> MSHHHHHHVSKIFFEQGTYQCLENCGTVALTIIRRGGDLTNTVFVDFRTEDGTANAGSDYEFTEGTVVFKPGETQKEIRVGIIDDDIFEEDKNFLVHLSNVKVSSEASEDGILEANHVSALACLGSPSTATVTIFDDDHAGIFTFEEPVTHVSESIGIMEVKVLRTSGARGNVIVPYKTIEGTARGGGEDF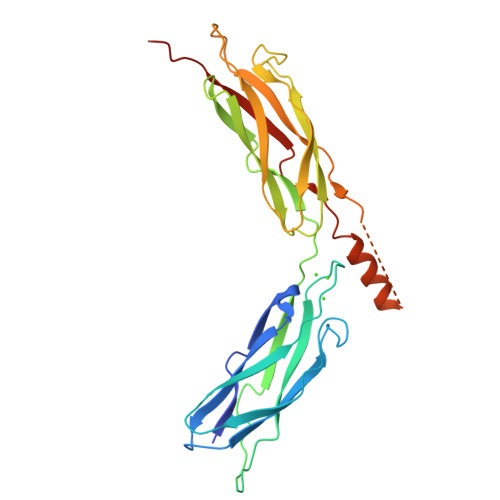EDTCGELEFQNDEIVKTISVKVIDDEEYEKNKTFFLEIGEPRLVEMSEKKGGFTITEEYDDKQPLTSKEEEERRIAEMGRPILGEHTKLEVIIEESYEFKSTVD> GPSSSKSEENISLVYEIDGTEALGSCLRVRPCSNDAPDLSKCTIQWYRSSSDGSKKELISGATKSVYAPEPFDVGRVLHADIIYDGHSLSLSTVGKIDPAAGLGSYVEALVRKHDVDFNVVVTQMSGEDHTSESIHLFHVGKMRIKLCKGKTVIAKEYYSSAMQLCGVRGGGNAAAQALYWQAKKGVSFVIAFESERERNAAIMLARRFACDCNVTLA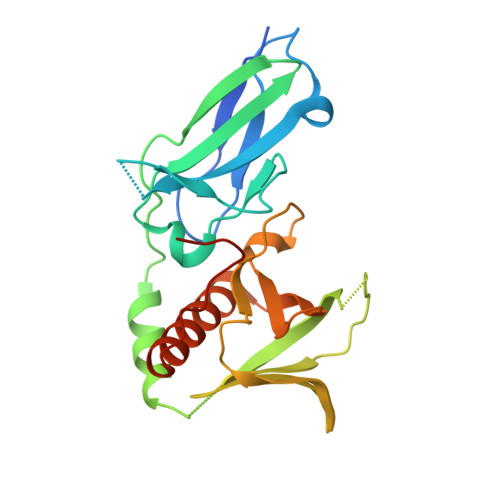GPEDRTETGQSP> MKVGQDKV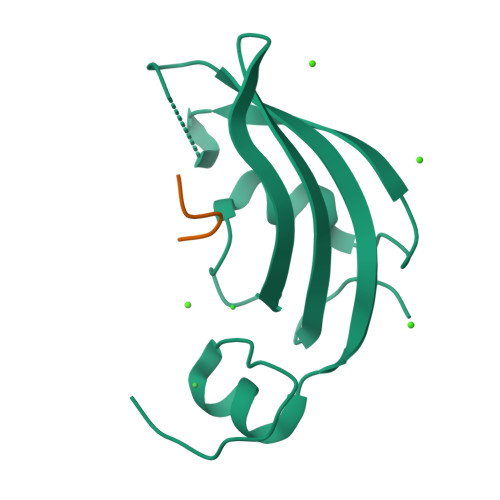VTIRYTLQVEGEVLDQGELSYLHGHRNLIPGLEEALEGREEGEAFQAHVPAEKAYGATGHPGIIPPHATLDFQVEVVKVREATPEELLHGHAHPSGHHHHHH;> TRYANPKMKPFIFGAX N6-methyladenosine (m6A) is the most abundant and prevalent internal modification in mRNA. In mammals, m6A exerts pivotal roles in posttranscriptional regulation and its dysregulation is implicated in various diseases including cancer. m6A is installed by a multicomponent methyltransferase complex (MTC, also known as the m6A writer complex). The mammalian MTC is composed of the core m6A methyltransferase METTL3–METTL14 complex (MTC core) and several regulatory proteins including WTAP, the adaptor responsible for METTL3–METTL14 localization and proper substrate recruitment, and VIRMA (KIAA1429), the specificity mediator that mediates preferential m6A modification at the 3′ untranslated regions (UTRs). WTAP and VIRMA are important subunits of the m6A writer complex.

We further purified the METTL3–METTL14–WTAP1–273–VIRMA381–1486 complex for gradient fixation and cryo-EM analysis. Unexpectedly, in the cryo-EM structure, only WTAP171–237 and VIRMA381–1292 (with the stoichiometric ratio 2:1) and an unassigned density close to WTAP were observed. The observed WTAP171–237–VIRMA381–1292 in the quaternary complex adopted a flag-and-pole-like architecture with dimensions of ~116 Å × 103 Å × 80 Å. Two WTAP171–237 molecules (designated WTAPA and WTAPB) formed an asymmetric homodimer (the “flag pole”) while VIRMA381–1292 that contains 17 armadillo-like (ARML) repeats (designated ARML 1–17) formed a twisted α-solenoid-like superhelix (the “flag”). Two long helices in between of ARML 4–5 and of ARML 7–8 mediate the turning of the VIRMA α-solenoid, possibly accounting for the formation of the twisted architecture. However, compared to the WTAPs alone, VIRMA-bound WTAPs bent around the observed N-termini (around WTAPA residue 188 and WTAPB residue 185) and displayed a more compact and dense conformation with distinct intramolecular interactions. Hydrogen bond interactions were also observed between WTAP Q201A side chain and K198B main chain and between N205A main chain and Q201B side chain. These together contributed to the formation of the compact VIRMA-bound WTAP dimer that harbors a contiguous negatively charged surface patch involved in the interaction with VIRMA. Three intermolecular interaction interfaces, designated Interfaces 1, 2, and 3, could be observed between the WTAP171–237 dimer and VIRMA381–1292 with buried areas of ~773.9 Å2, ~1155.6 Å2, and ~101 Å2, respectively. Interface 1 is located in between WTAPA (residues 205–224) and VIRMA (residues 452–660). Interfaces 2 and 3 are in between of WTAPB (residues 177–200, 214–221) and VIRMA (residues 657–1030, 494–497).

> MASVKLTELLDLYREDRGAKWVTALEEIPSLIIKGLSYLQLKNTKQDSLGQLVDWTMQALNLQVALRQPIALNVRQLKAGTKLVSSLAECGAQGVTGLLQAGVISGLFELLFADHVSSSLKLNAFKALDSVISMTEGMEAFLRGRQNEKSGYQKLLELILLDQTVRVVTAGSAILQKCHFYEVLSEIKRLGDHLAEKTSSLPNHSEPDHDTDAGLERTNPEYENEVEASMDMDLLESSNISEGEIERLINLLEEVFHLMETAPHTMIQQPVKSFPTMARITGPPERDDPYPVLFRYLHSHHFLELVTLLLSIPVTSAHPGVLQATKDVLKFLAQSQKGLLFFMSEYEATNLLIRALCHFYDQDEEEGLQSDGVIDDAFALWLQDSTQTLQCITELFSHFQRCTASEETDHSDLLGTLHNLYLITFNPVGRSAVGHVFSLEKNLQSLITLMEYYSKEALGDSKSKKSVAYNYACILILVVVQSSSDVQMLEQHAASLLKLCKADENNAKLQELGKWLEPLKNLRFEINCIPNLIEYVKQNIDNLMTPEGVGLTTALRVLCNVACPPPPVEGQQKDLKWNLAVIQLFSAEGMDTFIRVLQKLNSILTQPWRLHVNMGTTLHRVTTISMARCTLTLLKTMLTELLRGGSFEFKDMRVPSALVTLHMLLCSIPLSGRLDSDEQKIQNDIIDILLTFTQGVNEKLTISEETLANNTWSLMLKEVLSSILKVPEGFFSGLILLSELLPLPLPMQTTQVIEPHDISVALNTRKLWSMHLHVQAKLLQEIVRSFSGTTCQPIQHMLRRICVQLCDLASPTALLIMRTVLDLIVEDLQSTSEDKEKQYTSQTTRLLALLDALASHKACKLAILHLINGTIKGDERYAEIFQDLLALVRSPGDSVIRQQCVEYVTSILQSLCDQDIALILPSSSEGSISELEQLSNSLPNKELMTSICDCLLATLANSESSYNCLLTCVRTMMFLAEHDYGLFHLKSSLRKNSSALHSLLKRVVSTFSKDTGELASSFLEFMRQILNSDTIGCCGDDNGLMEVEGAHTSRTMSINAAELKQLLQSKEESPENLFLELEKLVLEHSKDDDNLDSLLDSVVGLKQMLES;>MHHHHHHHHHHSGDEVDAGSGHMTNEEPLPKKVRLSETDFKVMARDELILRWKQYEAYVQALEGKYTDLNSNDVTGLRESEEKLKQQQQESARRENILVMRLATKEQEMQECTTQIQYLKQVQQPSVAQLRSTMVDPAINLFFLKMKGELEQTKDKLEQAQNELSAWKFTPDSQTGKKLMAKCRMLIQENQELGRQLSQGRIAQLEAELALQKKYSEELKSSQDELNDFIIQLDEEVEGMQSTILVLQQQLKETRQQLAQYQQQQSQASAPSTSRTTASEPVEQSEATSKDCSRL[2x]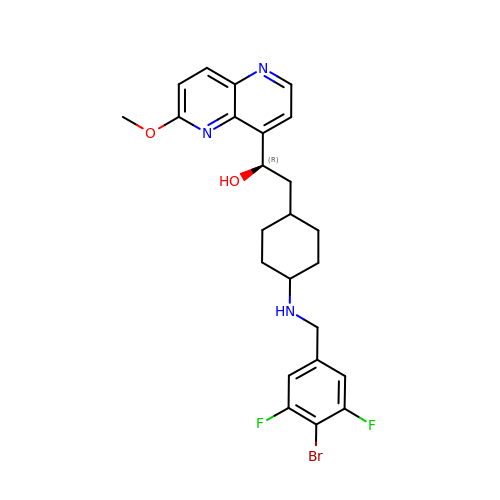(1~{R})-2-[4-[[4-bromanyl-3,5-bis(fluoranyl)phenyl]methylamino]cyclohexyl]-1-(6-methoxy-1,5-naphthyridin-4-yl)ethanol | C24 H26 Br F2 N3 O2 | RCLQISQKEHCDJQ-IUSZMWJPSA-N> GHMEQTHRAIFRFVP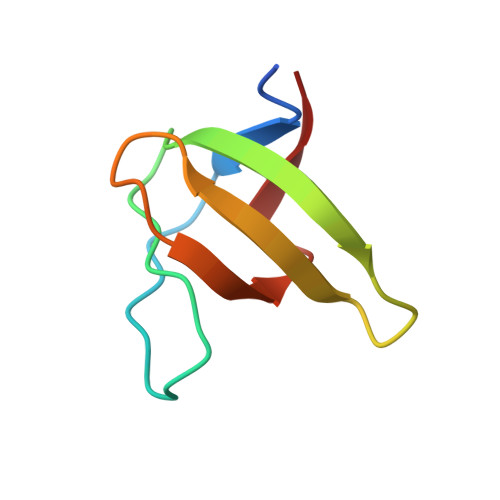RHEDELELEVDDPLLVELQAEDYWYEAYNMRTGARGVFPAYYAIEV> GSTMHTDGDKAFVDFLSDEIKEERKIQKHKTLPKMSGGWELELNGTEAKLVRKVAGEKITVTFNINNSGGSTPNFVVEVIKNDDGKKALVLDCHYGDIFSIREVSFQSTGESEWKDTNYTLNTDSLDWALYDHLMDFLADRGVDNTFADELVELSTALEHQEYI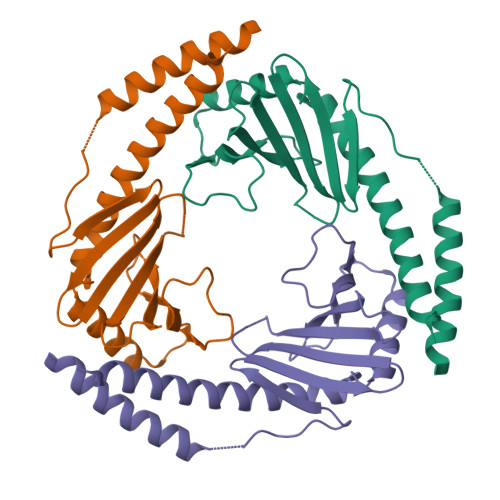TFLEDLKSFVKSQ>MANGVIPPPGGASPLPQVRVPLEEPPLSPDVEEEDDDLGKTLAVSRFGDLISKPPAWDPEKPSRSYSERDFEFHRHTSHHTHHPLSARLPPPHKLRRLPPTSARHTRRKRKKEKTSAPPSEGTPPIQEEGGAGVDEEEEEEEEEEGESEAEPVEPPHSGTPQKAKFSIGSDEDDSPGLPGRAAVTKPLPSVGPHTDKSPQHSSSSPSPRARASRLAGEKSRPWSPSASYDLRERLCPGSALGNPGGPEQQVPTDEAEAQMLGSADLDDMKSHRLEDNPGVRRHLVKKPSRTQGGRGSPSGLAPILRRKKKKKKLDRRPHEVFVELNELMLDRSQEPHWRETARWIKFEEDVEEETERWGKPHVASLSFRSLLELRRTIAHGAALLDLEQTTLPGIAHLVVETMIVSDQIRPEDRASVLRTLLLKHSHPNDDKDSGFFPRNPSSSSMNSVLGNHHPTPSHGPDGAVPTMADDLGEPAPLWPHDPDAKEKPLHMPGGDGHRGKSLKLLEKIPEDAEATVVLVGCVPFLEQPAAAFVRLNEAVLLESVLEVPVPVRFLFVMLGPSHTSTDYHELGRSIATLMSDKLFHEAAYQADDRQDLLSAISEFLDGSIVIPPSEVEGRDLLRSVAAFQRELLRKRREREQTKVEMTTRGGYTAPGKELSLELGGSEATPEDDPLRRTGRPFGGLIRDVRRRYPHYLSDFRDALDPQCLAAVIFIYFAALSPAITFGGLLGEKTQDLIGVSELIMSTALQGVVFCLLGAQPLLVIGFSGPLLVFEEAFFSFCSSNHLEYLVGRVWIGFWLVFLALLMVALEGSFLVRFVSRFTQEIFAFLISLIFIYETFYKLVKIFQEHPLHGCSASNSSEVDGGENMTWAGARPTLGPGNRSLAGQSGQGKPRGQPNTALLSLVLMAGTFFIAFFLRKFKNSRFFPGRIRRVIGDFGVPIAILIMVLVDYSIEDTYTQKLSVPSGFSVTAPEKRGWVINPLGEKSPFPVWMMVASLLPAILVFILIFMETQITTLIISKKERMLQKGSGFHLDLLLIVAMGGICALFGLPWLAAATVRSVTHANALTVMSKAVAPGDKPKIQEVKEQRVTGLLVALLVGLSIVIGDLLRQIPLAVLFGIFLYMGVTSLNGIQFYERLHLLLMPPKHHPDVTYVKKVRTLRMHLFTALQLLCLALLWAVMSTAASLAFPFILILTVPLRMVVLTRIFTDREMKCLDANEAEPVFDEREGVDEYNEMPMPV[2x]

Anion exchanger 3 (AE3) is pivotal in regulating intracellular pH across excitable tissues, yet its structural intricacies and functional dynamics remain underexplored compared to other anion exchangers. This study unveils the structural insights into human AE3, including the cryo-electron microscopy structures for AE3 transmembrane domains (TMD) and a chimera combining AE3 N-terminal domain (NTD) with AE2 TMD (hAE3NTD2TMD). Our analyzes reveal a substrate binding site, an NTD-TMD interlock mechanism, and a preference for an outward-facing conformation. Unlike AE2, which has more robust acid-loading capabilities, AE3’s structure, including a less stable inward-facing conformation due to missing key NTD-TMD interactions, contributes to its moderated pH-modulating activity and increased sensitivity to the inhibitor DIDS.

To overcome this obstacle and gain structural insight into the AE3 NTD, we constructed a chimeric anion exchanger, combining the NTD of hAE3 (297–671) with the TMD of hAE2 (672–1241). This chimera, termed hAE3NTD2TMD, was designed to exhibit the inward-facing conformation with a visible NTD, capitalizing on the thermostability of human AE2’s inward-facing state. Functional assays in HEK293 cells confirmed the pH-mediating activities of the hAE3NTD2TMD chimera, and both 2D and 3D-classifications displayed EM signals indicative of a full-length anion exchanger. The cryo-EM structure of hAE3NTD2TMD was determined at an overall resolution of 3.35 Å, with both AE3 NTD and AE2 TMD clearly resolved in the EM map. In the hAE3NTD2TMD structure, similar to the full-length human AE2 structure, a homodimer formation is observed where the TMDs adopt an inward-facing conformation. The AE3 NTD comprises seven β-strands (a-g) arranged in a planar configuration, sandwiched by eight helices (NH1-8). Dimerization of the AE3 NTDs is primarily facilitated by interactions among the loops linking NH7/8 (loopNH7/8) and NH1/β strand c (loopNH1/c), as well as helix NH8 from both protomers. In the hAE3NTD2TMD structure, the AE3 NTD engages with the AE2 TMD in a manner reminiscent of AE2’s own NTD-TMD interactions, with the loopTMH10/11 extending from the TMD into the NTD surface. Specifically, substituting Q618AE2 with E617AE3 disrupts the original contact between Q618AE2 and D1079AE2 in AE2. This results in a new electrostatic interaction between E617AE3 and K1080AE2 in the hAE3NTD2TMD chimera. In our structure of the NTDAE3-TMDAE2 chimera, densities of PIP2, cholesterol, and CHS in the TMD of AE2 correspond with the previous AE1 and AE2 models, further confirming the lipid regulation of human AE2.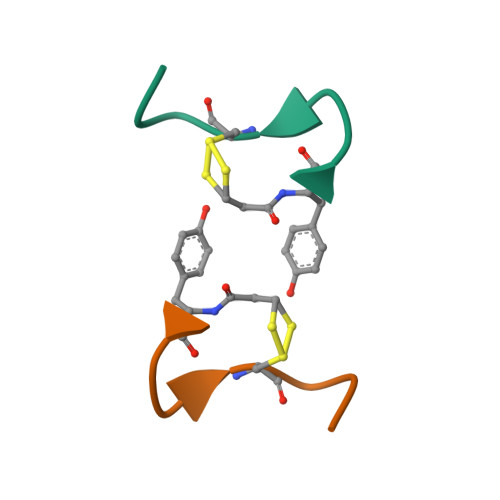>[2x]XYIQNCPLGX N-propan-2-ylurea | C4 H10 N2 O | 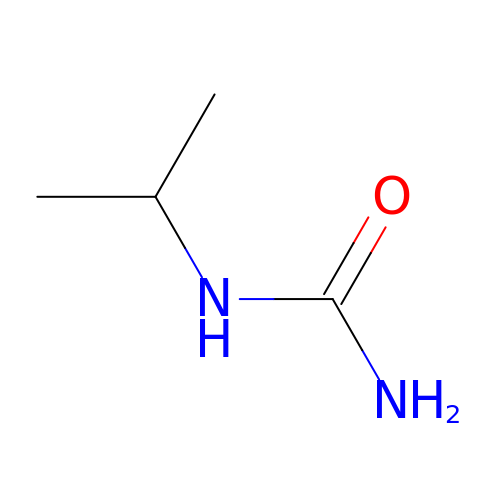LZMATGARSSLFMQ-UHFFFAOYSA-N> MLKRFPTPILKVYWPFFVAGAAVYYGMSKAADLSSNTKEFI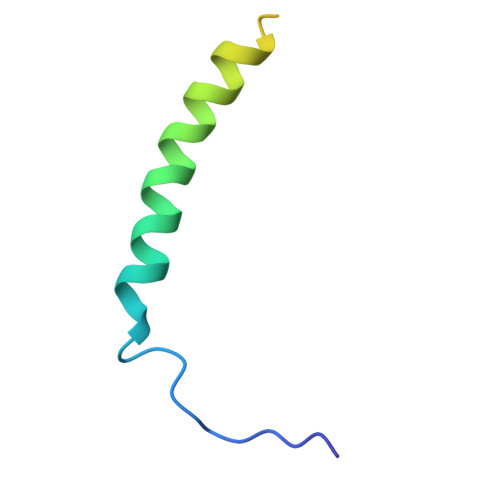NDPRNPRFAKGGKFVEVD>MASSLLTSSGIIPTTGSNMVVRSFLPFGSVRLTRPYNNSSLLISCCSSVSKNAETSGTDLKTIVERWPEYIPNKLPDKNYVRVFDTTLRDGEQSPGAALTPPQKIEIARQLAKLRVDIMEVGFPVSSEEEFETIQTIAKTVGNEVDEETGYIPVICVIARSKERDIKAAWESVKYAKRPRIVIFTSTSDIHLKYKLKMTREEVVDMVASSIRFAKSLGFEDIEFGCEDGGRSDKDYICTVFEEAIKAGATTLACPDTVGINMPHEYGKLVRYIKANTPGIDDVIFSAHCHNDLGVATANTIAGICAGAR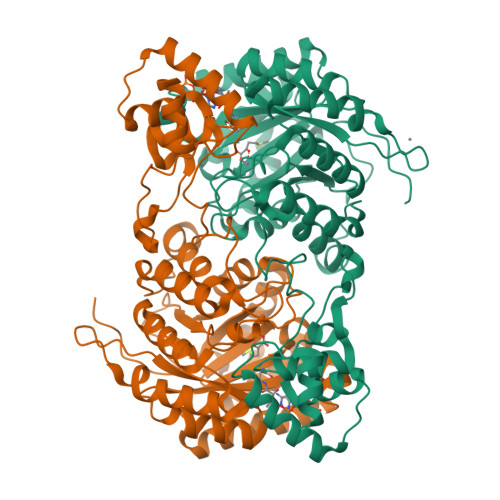QVEVTINGIGERSGNAPLEEVVMALKCRGAFVMGGVYTRIDTRQIMATSKMVQEYTGLYVQPHKPIVGANCFVHESGIHQDGILKNRSTYEIISPEDVGVVKSQNSGIVLGKLSGRHAVKGRLKELGYEISDEKLNEVFSRFRDLTKQKKRVTDDDLKALVTCGDEIFSSDKLNGTDDNEINSNGYVPAPQISSVV[2x]> GSQQRKVLTLEKG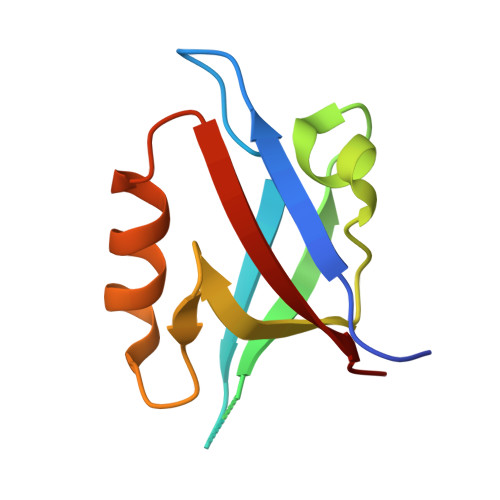DNQTFGFEIQTYGLHHREEQRVEMVTFVARVHESSPAQLAGLTPGDTIASVNGLNVEGIRHREIVDIIKASGNVLRLETLYGT>[2x]APEPPSADYASLVDVFVGTEGDFGNDMPAAQAPNGLAKVNPRTTPGRNNTGYDYAQSKISGFTHTNLDGVGGSGGGGDLLVVPTSGSYTARPGTGTYAHPFSHDDEDAGPGFYSVGLGNVAGTDGAITGAPGTIEAEVAAATRSGVHRYAFPAGSTPSLVVDLETNNTSRRSSSVQVETRADGTVELSGQVTGYFYNAAYTLYYTARTLQPATVQTWGDDDRLVDATAQDGVDTGAILTFDPADAGEIGLQVTLSPVSVEQARIDQQVELGDLSFDAIRDRTRAEWNATLGRVAIDASTATDPTGELQRLFY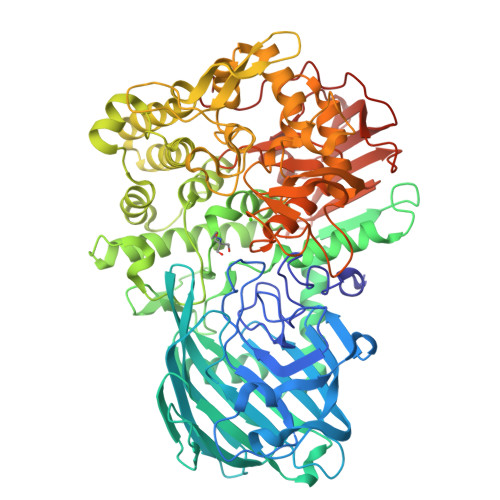THLYRMFAMPMNATSTSGTYRGVDGAVHAAQGFTYYDSWATWDDFRKFSVIAYIDPALYRDMVQSLVYLFADAEATGTGGGLGGFVHSVPTVRWERSSVVVADAIAKGFDGFDRLDEAYPALQRLVGQYSADELRRGYVAGNPGASVQRGYDQYGLSVIADELGLTEEAETLREQASWPIEKLTKPGAWTAADGTQVGLLTPRAADGSWQSADHAKFEAAGLYQGTLWQYHWYDAYDMDALVEAMGGHEAARLGMRHMFGEHAPDDGKAMLHSNANEIDLQAPYLFNYTGEPSLTQKWARAIYTKETWNRYIATGSSSAVPSGGGEFTPPLKTKVYRLDPRGMLPTMDNDAGTMSTMFVAAAVGLFPVTAGSSQFQVGSPFFDSTTITYDDGSAFTVTADGVSEDAFYVQSATLDGATFGNTWVDYATVVGGADLAFRMGEQPSDWGTDTAPAFSMSTATDE> MAPGSKTELRSVTNGQSNQPSNEGDAIKVFVRIRPPAERSGSADGEQNLSLSVLSSTSLRLHSNPEPKTFTFDHVADVDTTQESVFATVAKSIVESCMSGYNGTIFAYGQTGSGKTFTMMGPSESDNFSHNLRGVIPRSFEYLFSLIDREKEKAGAGKSFLSKCSFIEIYNEQIYDLLDSASAGLYLREHIKKGVFVVGAVEQVVTSAAEAYQVLSGGWRNRRVASTSMNRESSRSHAVFTITIESMEKC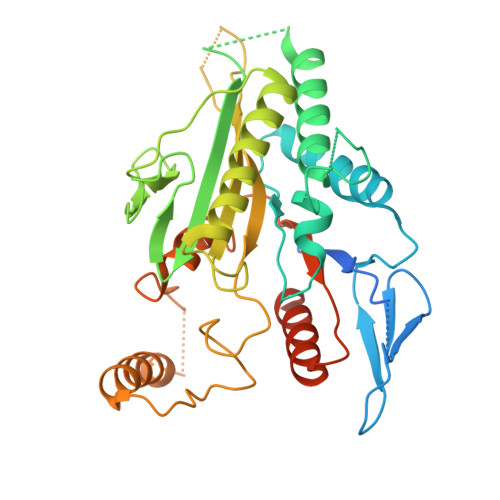NEIVNIRTSLLNLVDLAGSERQKDTHAEGMRLKEAGNINRSLSTLGQVITALVDVGNGKQRHVSYRDSKLTFLLRDSLGGNAKTAIIANVHPGSRSFGETLSTLNFAQRAKLIKNKAVVNEDTQCLEHHHHHH> MSALSLLILG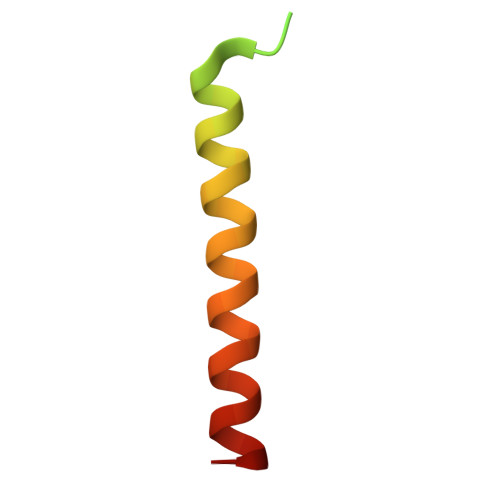LLTAVPPASCQQGLGNLQPWMQGLIAVAVFLVLVAIAFAVNHFWCQ>[4x]GSMEKAAVNEDGLVIPLIDFSKFLEGDETLKLETAKAILHGFQTAGFIYLKNIPIQPDFREHVFNTSAKFFKLPKEKKLEVGWTTPEANRGYSAPGREKVTQLTDPAEIEKIRSAAPDIKESYEIGREDEPGHPNPWPAEQDDLVGFKSTMNNFFDQCKALHIEVMRAIAVGMGIDANYFDSFVDVGDNI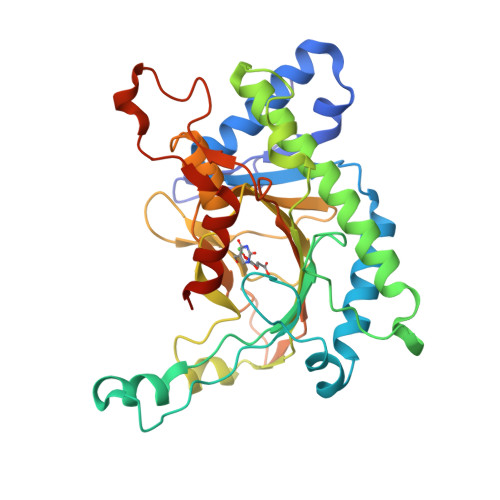LRLLHYPAVKSEVFKINPGQVRAGEHTDYGSITLLFQDSRGGLQVKSPNGQFIDATPIENTVVVNAGDLLARWSNDTIKSTVHRVVEPPKQEDVHPPRYSIAYFCNPNHKSYIEAIPGTYAAESERKYEGINSGKYLVQRLAATYLEHHHHHH> MAAA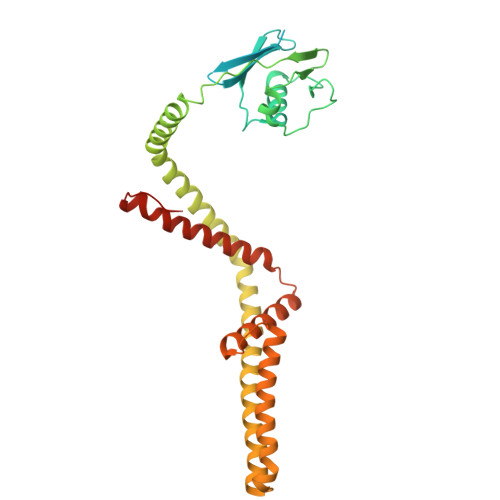AGRSLLLLLSSRGGGGGGAGGCGALTAGCFPGLGVSRHRQQQHHRTVHQRIASWQNLGAVYCSTVVPSDDVTVVYQNGLPVISVRLPSRRERCQFTLKPISDSVGVFLRQLQEEDRGIDRVAIYSPDGVRVAASTGIDLLLLDDFKLVINDLTYHVRPPKRDLLSHENAATLNDVKTLVQQLYTTLCIEQHQLNKERELIERLEDLKEQLAPLEKVRIEISRKAEKRTTLVLWGGLAYMATQFGILARLTWWEYSWDIMEPVTYFITYGSAMAMYAYFVMTRQEYVYPEARDRQYLLFFHKGAKKSRFDLEKYNQLKDAIAQAEMDLKRLRDPLQVHLPLRQIGEKD>MEADVEQQALTLPDLAEQFAPPDIAPPLLIKLVEAIEKKGLECSTLYRTQSSSNLAELRQLLDCDTPSVDLEMIDVHVLADAFKRYLLDLPNPVIPAAVYSEMISLAPEV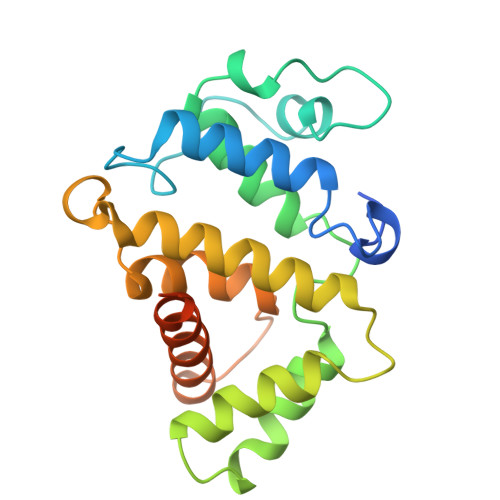QSSEEYIQLLKKLIRSPSIPHQYWLTLQYLLKHFFKLSQTSSKNLLNARVLSEIFSPMLFRFSAASSDNTENLIKVIEILISTEWNERQPAPALPPKPPKPTTVAN[2x]>MGKGHHHHHHGSERTGTQPLGVQGLTEEQRMMIRELMDAQMKTFDTTFSHFKNFRLPGVLSSGCELPESLQAPSREEAAKWSQVRKDLCSLKVSLQLRGEDGSVWNYKPPADSGGKEIFSLLPHMADMSTYMFKGIISFAKVISYFRDLPIEDQISLLKGAAFELCQLRFNTVFNAETGTWECGRLSYCLEDTAGGFQQLLLEPMLKFHYMLKKLQLHEEEYVLMQAISLFSPDRPGVLQHRVVDQLQEQFAITLKSYIECNRPQPAHRFLFLKIMAML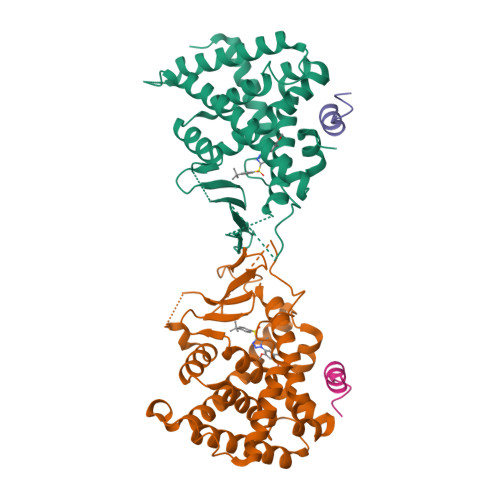TELRSINAQHTQRLLRIQDIHPFATPLMQELFGITGS[2x];>CPSSHSSLTERHKILHRLLQEGSPS[2x]>MAILGLGTAIVEIARIEAVIARSGDRLARRVLSDNEWAIWKTHHQPVRFLAKRFAVKEAAAKAFGTGIRNGLAFNQFEVFNDELGKPRLRLWGEALKLAEKLGVANMH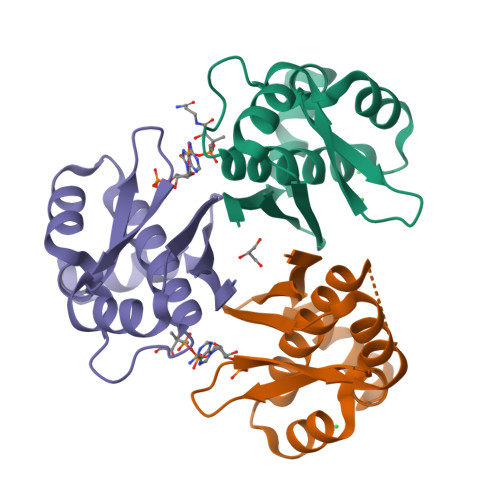VTLADERHYACATVIIES[3x]> HMSKVPRNFRLLEELEKGEKGFGPESCSYGLADSDDITMTKWNGTILGPPHSNHENRIYSLSIDCGPNYPDSPPKVTFISKINLPCVNPTTGEVQTDFHTL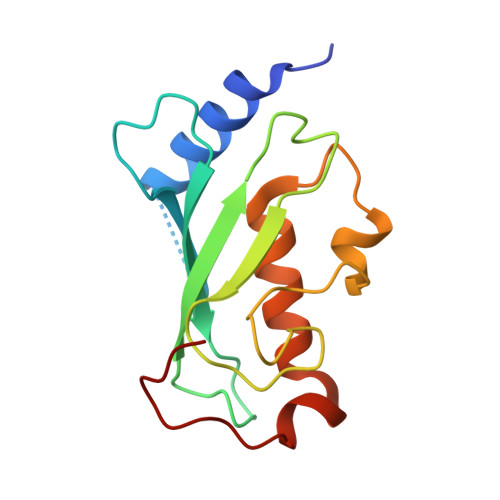RDWKRAYTMETLLLDLRKEMATPANKKLRQPKEGETF> GPGSSRWSKDYDVCVCHSEENLVAAQDLVSYLEGSTASLRCFLQLRDATPGGAIVSELCQALSSSHCR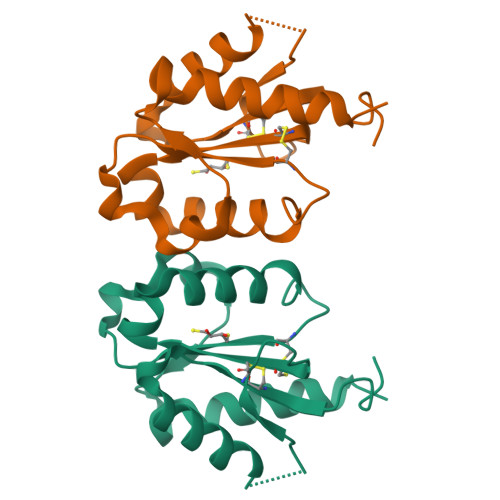VLLITPGFLQDPWCKYQMLQALTEAPGAEGCTIPLLSGLSRAAYPPELRFMYYVDGRGPDGGFRQVKEAVMRYLQTLS> SNAQYEDGKQYTTLEKPVAGAPQVLEFFSFFCPHAYQFEEVLHISDNVKKKLPEGVKMTKYHVNFMGGDLGKDLTQAWAVAMALGVEDKVTVPLFEGVQKTQTIRSASDI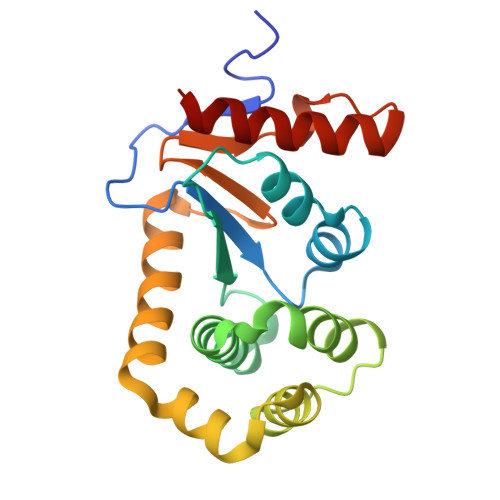RDVFINAGIKGEEYDAAWNSFVVKSLVAQQEKAAADVQLRGVPAMFVNGKYQLNPQGMDTSNMDVFVQQYADTVKYLSEKK>MTKQEKTALNMAR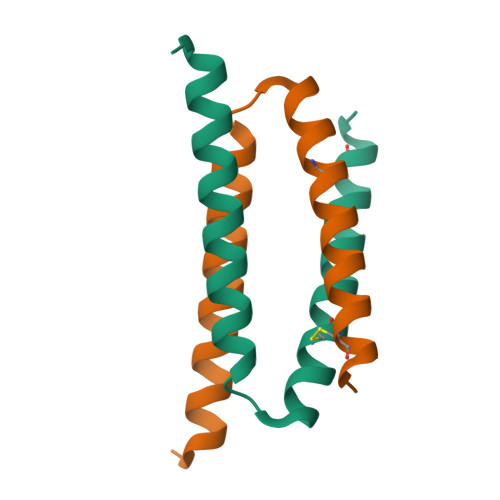FIRSQTLTLLEKLNELDPDEQADICESLHDHADELYRSCLARFGDDGENL[2x]> MENTENSVDSKSIKNLEPKIIHGSESMDSGISLDNSYKM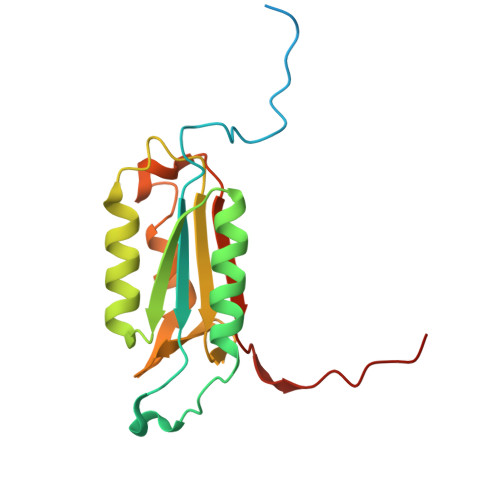DYPEMGLCIIINNKNFHKSTGMTSRSGTDVDAANLRETFRNLKYEVRNKNDLTREEIVELMRDVSKEDHSKRSSFVCVLLSHGEEGIIFGTNGPVDLKKITNFFRGDRCRELTGKPKLFIIQACRGTELDCGIETD>[2x]GPHMKRYNVITIFPEMINEIFKYGVLSKGIDIGLFRVNPINLRDYTEDKHKTVDDYQYGGGHGLVMKPEPIYKAIADLKSKKDTHVVFLDPRGEQFTQKTAERLYNYDDITFVCGRYEGIDDRVRELMADEMISIGDFVITGGELAAVTIIDAVARLIPGVLGDENSPNEESFTTGLLEYPHFTRPAEFMGKKVPEVLISGNHEEIRRWRLTESIKTTLQNRPDMILRKSLSREEEQILWSLTRGVQRKYNIYVALMHYPMRDKEGKVVTTSITNMDLHDISRSCRTFGVKNYFVVNPMPAQREIASRVVRHWIKGYGATYNENRKEAFEYTIITDSLASVIKSIEEKESGSPIIIATTARYQQKAISIEKLKEIADRPILLLFGTGWGFVDDILEFADYVLKPIHGVGDFNHLSVRSAVAIYLDRINRSFQEDIL

Using both theoretical and experimental approaches we studied in detail TrmD-Tm1570—a fusion between TrmD and Tm1570 proteins found in 66 organisms. Within the PF01746 family, there is a well-studied TrmD protein that modifies the N1 position of G37 in tRNA. In the PF01746-PF09936 architecture, TrmD is fused with Tm1570. The Tm1570 protein belongs to the SAM-dependent RNA MT family (Pfam ID: PF09936).

Our theoretical and experimental analysis shows that the CnTrmD-Tm1570 protein functions as a homodimer, unlike other double knotted proteins we study here. Therefore, we used AlphaFold Multimer to model the structure and obtained a compact homodimeric complex with the main interchain interactions present between the corresponding domains. Both of the domains interact in a standard fashion (antiparallel for TrmD and perpendicular for Tm1570) with their counterparts from the other chain. Herein, based on our analysis of structure and sequence, we found that deep trefoil knots provide the binding sites for SAM in both the TrmD and Tm1570 domains of the fusion. Based on C. nitroreducens we established that the protein is a homodimer capable of binding four ligands (S-adenosylmethionine)—one in each knotted binding site, and a single tRNA molecule (based on the similarities with HiTrmD). The SGHH motif (residues 198–201 in HiTrmD) that interacts with G37 in the substrate tRNAs for the methylation process is present in SGNH form in the C. nitroreducens fusion. With respect to the native C. nitroreducens tRNA Leu (CAG) substrate, the TrmD domain retained 86% ± 4% activity of the fusion protein, while Tm1570 retained only 18% ± 9%. These data clearly demonstrate that the enzymatic activity of the fusion TrmD-Tm1570 protein towards tRNA Leu (CAG) substrate is governed by the TrmD domain. However, based on structural similarities, we believe that it also acts as a tRNA MT, probably by modifying 2’O in ribose. Our model and the crystal structure are similar, in particular, both of them show “open” domain organization that enables homodimer formation.N-[(1S,5R)-3-(5-fluoro-2-{[1-(2-hydroxyethyl)-1H-pyrazol-4-yl]amino}pyrimidin-4-yl)-3-azabicyclo[3.1.0]hexan-1-yl]cyclopropanecarboxamide 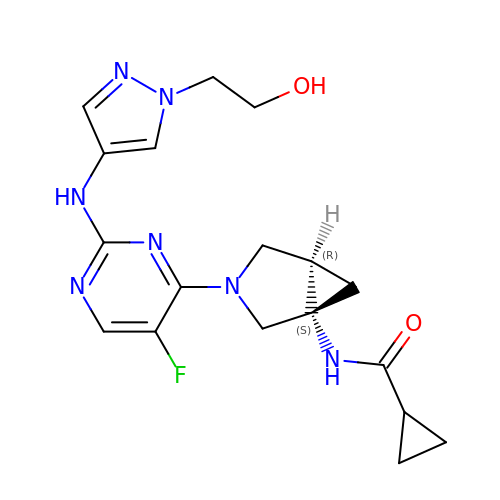| C18 H22 F N7 O2 | GYRPAYDYHMZXQT-KZULUSFZSA-N>SNAGGSSPITGLVYDQRMMLHHNMWDSHHPELPQRISRIFSRHEELRLLSRCHRIPARLATEEELALCHSSKHISIIKSSEHMKPRDLNRLGDEYNSIFISNESYTCALLAAGSCFNSAQAILTGQVRNAVAIVRPPGHHAEKDTACGFCFFNTAALTARYAQSITRESLRVLIVDWDVHHGNGTQHIFEEDDSVLYISLHRYEDGAFFPNSEDANYDKVGLGKGRGYNVNIPWNGGKMGDPEYMAAFHHLVMPIAREFAPELVLVSAGFDAARGDPLGGFQVTPEG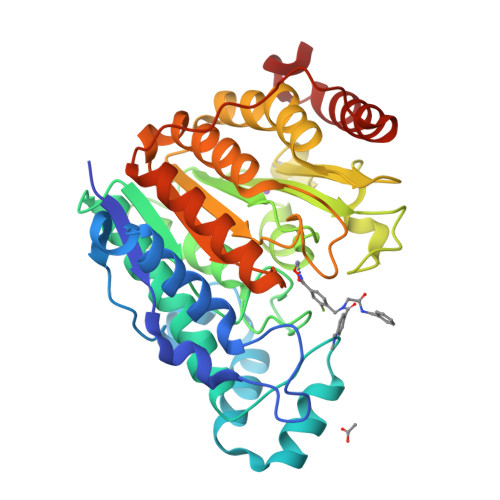YAHLTHQLMSLAAGRVLIILEGGYNLTSISESMSMCTSMLLGDSPPSLDHLTPLKTSATVSINNVLRAHAPFWSSLR[4x]>AAAAAAAA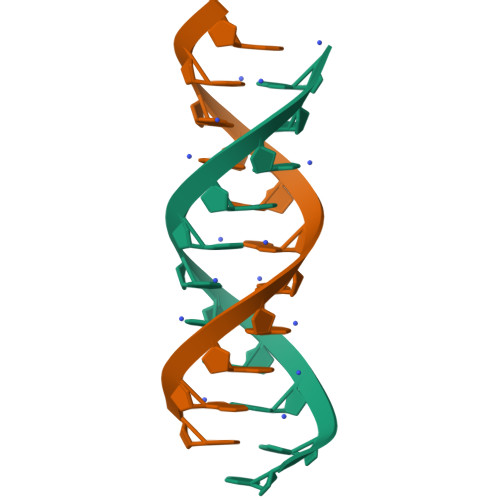AAA[2x]>QEGNGPAAVHYQPASPPRDACVYSSCYSEENVWKLCEYIKNHDQYPLEECYAVFISNERKMIPIWKQQARPGDGPVIWDYHVVLLHVSSGGQSFIYDLDTVLPFPCLFDTYVEDAIKSDDDIHPQFRRKFRVICADSYLKNFASDRSHMKDSSGNWREPPPPYPCIETGDSKMNLNDFISMDPKVGWGAVYTLSEFTHRFG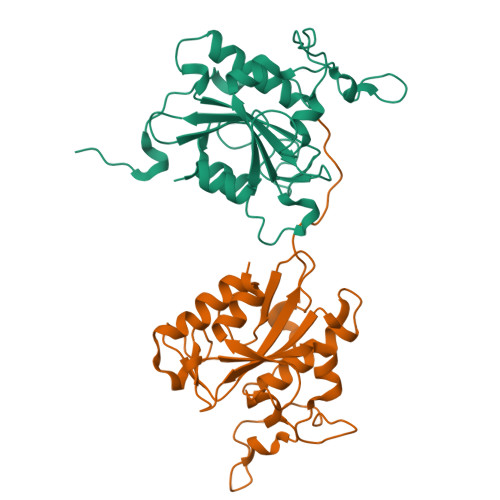S[2x]> MGHHHHHHMAPHTIPLPAAMRVQTGESGFSLKNGVRLPEKNPLSRQAERIFRDNGINTALVKNNADIIFTEDASLGREGYRLAVTPDSISIASGSVNGTLYALQSLVQSIAADKNGAPALPRMDVKDQPRFSWRGLMVDSCRHMMPVRDIKKVLDLMERYKFNTLHWH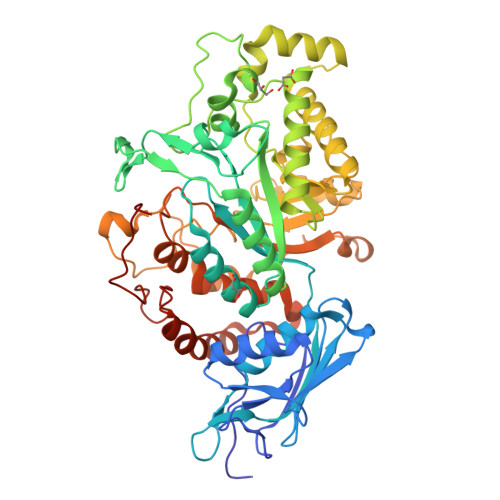LTDDQGWRLPIAKYPRLTTVGGARAQSPVIGNRNKGDGIPYSGHYTADEIRDVVRYARDRGITVIPEVEMPGHASAAIAAYPELGNTDIPGYEPRVQETWGVHSYTFSPTEKTFRFLEDVIDEICALFPDSPYIHIGGDEAPKNQWKQSPTAQRVMKDNGLANEHELQSYFIRRVEKMINNRGKRLIGWDEIQEGGLSPTATMMVWRSQMPHIAAQALAQGNDIVMTPNSHLYFDYDQGPGKPAAPEYETINNNQLTWQHVYGLEPVPQGTPREREKQVLGCQANIWTEYIPNLPKWEYHVFPRALALAEVAWTPQELKNEKDFRKRLDRQLPFLDARGVNYKRPDNGAPAQPKAVITRERRLEHHHHHH> MSGDENPASKPTPVQDVQGDGRWMSLHHRFVADSKDKEPEVVFIGDSAVQLMHQCEIWRELFSPLHALNFGIGGDSTQHVLWRLENGELEHIRPKIVVVWVGTNNHGHTAEQVTGGIKAIVQLVNERQPQARVVVL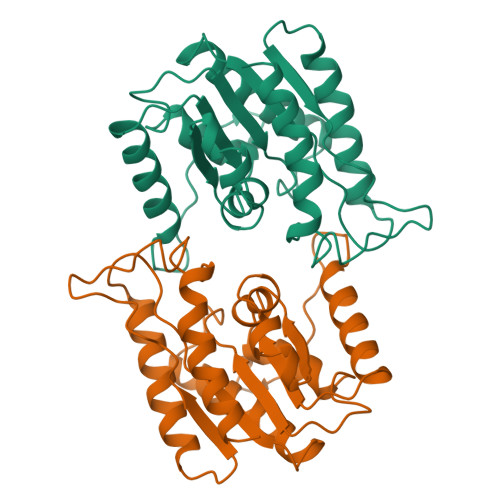GLLPRGQHPNPLREKNRRVNELVRAALAGHPRAHFLDADPGFVHSDGTISHHDMYDYLHLSRLGYTPVCRALHSLLLRLLTQDQGQGGAPLPEPSPP> AEETLMDSTTATAELGWMVHPPSGWEEVSGYDENMNTIRTYQVCNVFESSQNNWLRTKFIRRRGAHRIHVEM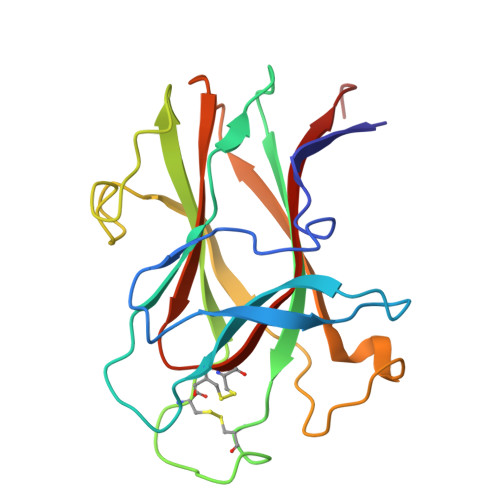KFSVRDCSSIPSVPGSCKETFNLYYYEADFDLATKTFPNWMENPWVKVDTIAADESFSQVDLGGRVMKINTEVRSFGPVSRNGFYLAFQDYGGCMSLIAVRVFYRKCPR> MSHGK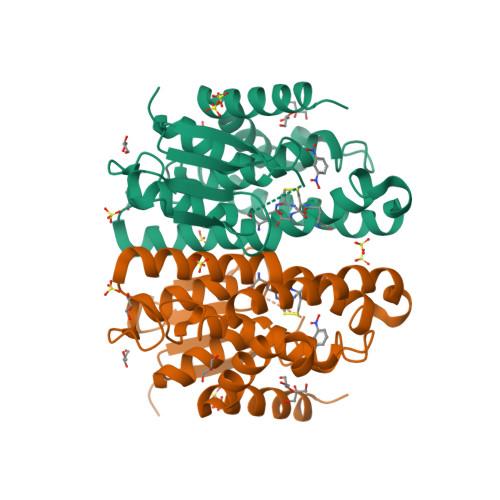QFTLFNHQVGPNGWKVDMLLRELGLSFETVYVNLGQREHKSPSFTKYNPNGRIPALIDHYYNDFVVWESDAILLYIVEKYDPEHKFSVSTFDDKIIMTQWLFFQASGQGPYFGQAGWFLAVAPPEERNPTIAERYQKEILRVFGVLESVLSQRQWLVADKLTIADISFVIWNATAVNLLVKGYKGFDFEKDFPSVHRWHTALITRPAIAESLKTKAEAIAQMNR>MGKSLSHLPLHSSKEDAYDGVTSENMRNGLVNSEVHNEDGRNGDVSQFPYVEFTGRDSVTCPTCQGTGRIPRGQENQLVALIPYSDQRLRPRRTKLYVMASVFVCLLLSGLAVFFLFPRSIDVKYIGVKSA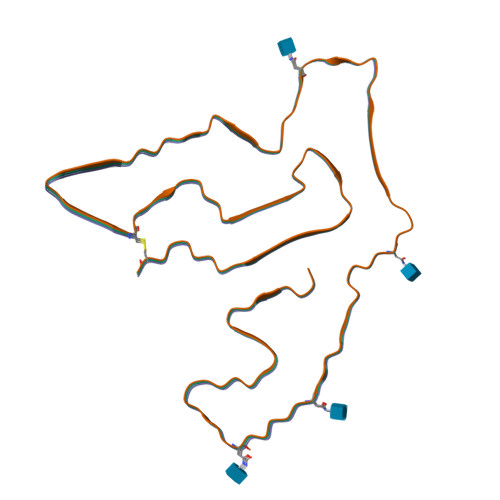YVSYDVQKRTIYLNITNTLNITNNNYYSVEVENITAQVQFSKTVIGKARLNNITIIGPLDMKQIDYTVPTVIAEEMSYMYDFCTLISIKVHNIVLMMQVTVTTTYFGHSEQISQERYQYVDCGRNTTYQLGQSEYLNVLQPQQ[3x]3-(1,3-thiazol-2-yl)propanoic 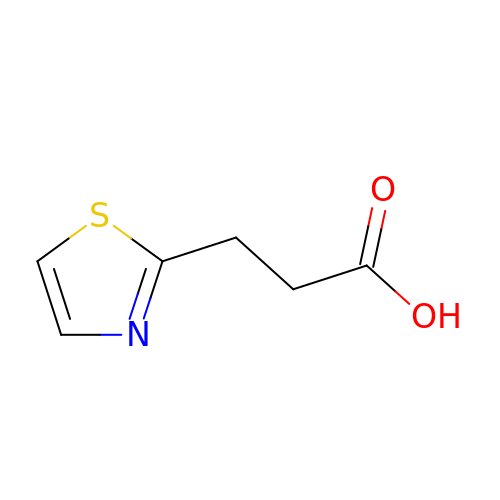acid | C6 H7 N O2 S | OJTQVDTVCPIZQH-UHFFFAOYSA-N> MDSISLRVALNDGNFIPVLGFGTTVPEKVAKDEVIKATKIAIDNGFRHFDSAYLYEVEEEVGQAIRSKIEDGTVKREDIFYTSKLWSTFHRPELVRTCLEKTLKST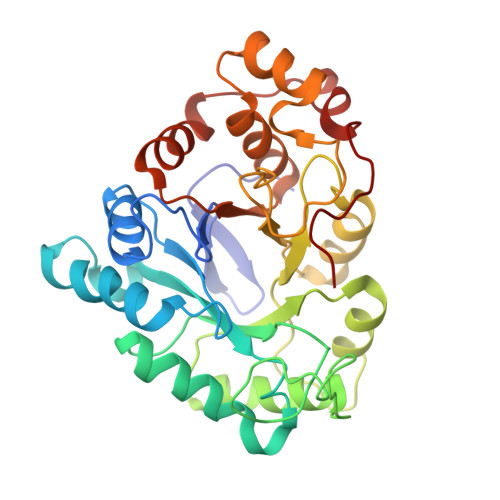QLDYVDLYIIHFPMALQPGDIFFPRDEHGKLLFETVDICDTWEAMEKCKDAGLAKSIGVSNFNCRQLERILNKPGLKYKPVCNQVECHLYLNQSKMLDYCKSKDIILVSYCTLGSSRDKTWVDQKSPVLLDDPVLCAIAKKYKQTPALVALRYQLQRGVVPLIRSFNAKRIKELTQVFEFQLASEDMKALDGLNRNFRYNNA> KSVIRWCTVSSPEEKKCNNLRDLTQQERISLTCVQKATYLDCIKAIANNEADAISLDGGQVFEAGLAPYKLKPIAAEVYEHTEGSTTSYYAVAVVKKGTEFTVNDLQGKTSCHTGLGRSAGWNIPIGTLIHRGAIEWEGIESGSVEQAVAKFFSASCVPGATIEQKLCRQCKGDPKTKCARNAPYSGYSGAFHCLKDGKGDVAFVKHTTVNENAPDQKDEYELLCLDGSRQPVDNYKTCN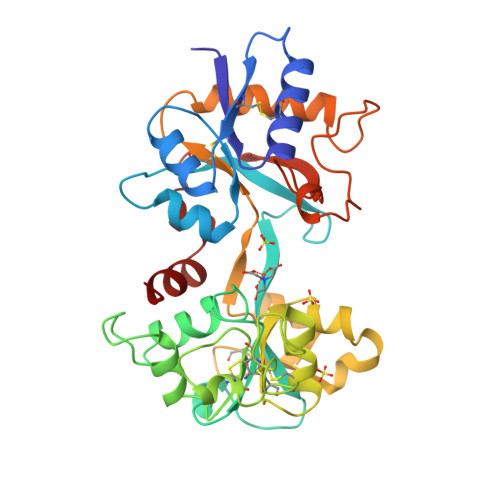WARVAAHAVVARDDNKVEDIWSFLSKAQSDFGVDTKSDFHLFGPPGKKDPVLKDLLFKDSAIMLKRVPSLMDSQLYLGFEYYSAIQSMR> MTMADLHD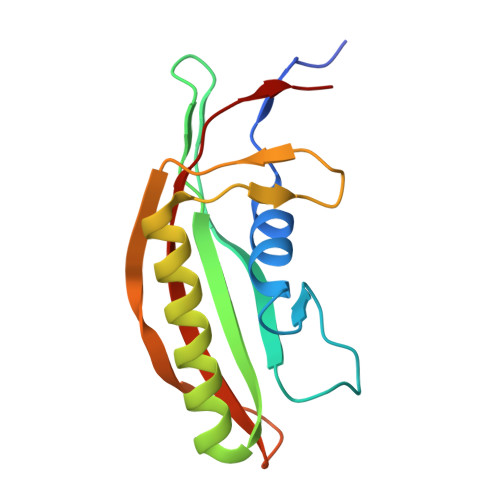QDAPDEEDFVVCWMQPVMRTAVERDIDAELPFCEVTRIDGADDPEAGTDDPVIQLDFYALGAEAAKAAAKQGHRRMLFLFRNFPTVTLSDGTLADLDFGETLIKPSRMAFEHDQIVRYTARYQLGTSYVAVP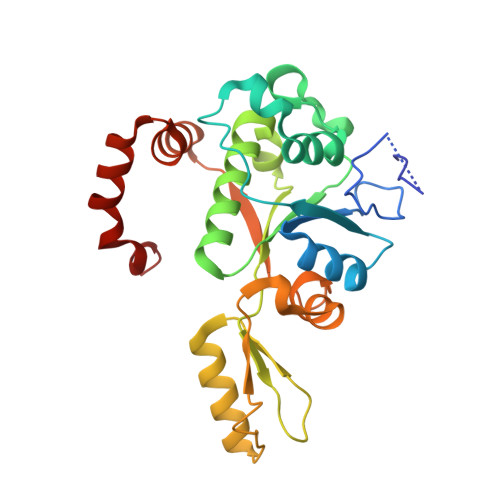> SNALVRRKSATDIGGLPGKLADCRSTDPRKSELYVVEGDSAGGSAKSGRDSMFQAILPLRGKIINVEKARIDRVLKNTEVQAIITALGTGIHDEFDIGKLRYHKIVLMADADVDGQHISTLLLTLLFRFMRPLIENGHVFLAQPPLYKLKWQRSDPEFAYSDRERDGLLEAGLKAGKKINKEDGIQRYKGLGEMDAKELWETTMDPSVRVLRQVTLDDAAAADELFSILMGEDVDARRSFITRNAKDVRFLDV>[2x]GSHMSTLKEVQDNITLHEQRLVTTRQKLKDAERAVELDP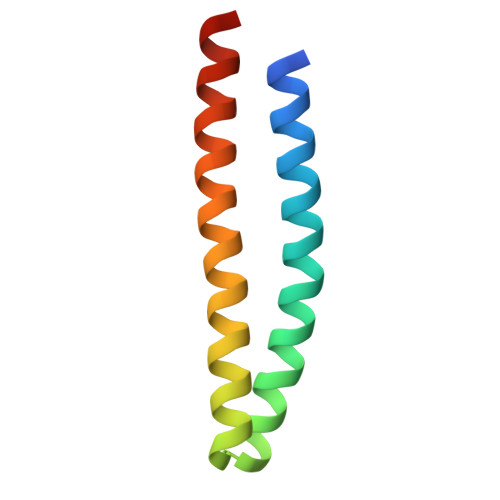DDVNKSTLQSRRAAVSALETKLGELKRELADLIAAQKLA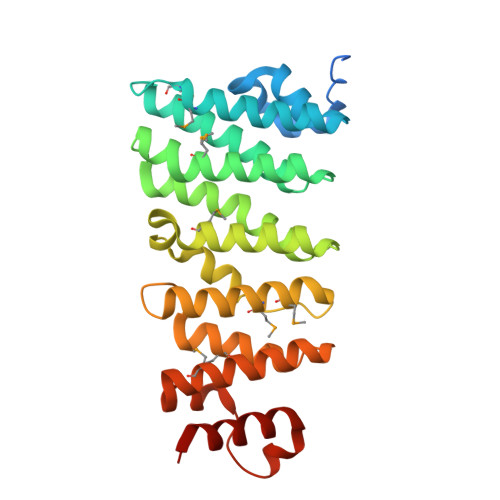>[2x]GPHGEAVVEPEMSNADISDARRGGMLGEPEPLTEKALREASSAIDVLGETLVAEAYCKTWSYREDALLALSKKLMEMPVGTPKEDLKNTLRASVFLVRRAIKDIVTSVFQASLKLLKMIITQYIPKHKLSKLETAHCVERTIPVLLTRTGDSSARLRVTAANFIQEMALFKEVKSLQIIPSYLVQPLKANSSVHLAMSQMGLLARLLKDLGTGSSGFTIDNVMKFSVSALEHRVYEVRETAVRIILDMYRQHQASILEYLPPDDSNTRRNILYKTIFEGFAKIDGRAT> LTFEHYWAQL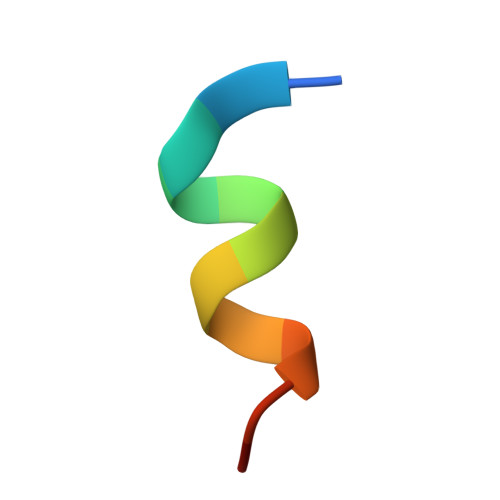TS In archaea, the 20S is composed of homo-heptameric α- and β-rings, and PAN (Proteasomal Activator Nucleotidase), a homohexamer proteasomal ATPase, is the RP found in many species. Unfolded substrates enter the chamber through a narrow pore in the center of α-rings, where N-termini of α-subunits form a gate to impede unregulated access to the proteolytic chamber. We designed and assembled in vitro various asymmetric archaea 20S, in which one of the two α-rings contains a point mutation, K66A, which prevents RP binding to the α-ring. Our studies reveal that, upon binding of a RP with a conserved C-terminal HbYX motif to one α-ring, the gate of the opposite α-ring opens allosterically, resulting in similar proteolytic activities of 20S singly capped and doubly capped with PAN.

The second activator is heptameric PA26 with the point mutation E102A and the last eight C-terminal residues replaced with the last eight C-terminal residues from PAN (with HbYX motif), which we named PA26PANc. The point mutation E102A abolishes a specific interaction between the so-called activation loop of PA26 with a reverse turn loop in the 20S α-subunit, thus abolishing the capability of PA26 to activate 20S proteasomes by opening its gate. Instead, the HbYX motif from the PAN C-terminus placed at the heptameric PA26PANc C-termini performs gate opening. PA26PANc activates the CP particle in the same manner as PAN, except that it symmetrically engages the 7-fold symmetric α-ring, and thus avoids a symmetry mismatch between the α-ring and the activator. We first determined the structure of PA26PANc-αWTββαK66A to resolutions of 2.9 Å without LFP substrate and 3.4 Å with LFP. In both our structures (with and without LFP), the distal α-ring, that without an activator, also shows features that match an open gate, with all N-termini moved away from the pore and pointing upwards. However, unlike the proximal gate, there is no rotation of distal α-subunits. Rather, the conformation of this α-ring matches well with that in the crystal structure of archaeal 20S proteasome in complex with PA26 (PDB: 1YAR20), except that the gate is in an open conformation. The surprising observation that binding of PA26PANc to the proximal α-ring opens the gate of the distal α-ring is consistent with allosteric action.

>[14x]TTTVGITLKDAVIMATERRVTMENFIMHKNGKKLFQIDTYTGMTIAGLVGDAQVLVRYMKAELELYRLQRRVNMPIEAVATLLSNMLNQVKYMPYMVQLLVGGIDTAPHVFSIDAAGGSVEDIYASTGSGSPFVYGVLESQYSEKMTVDEGVDLVIRAISAAKQRDSASGGMIDVAVITRKDGYVQLPTDQIESRIRKLGLIL;>AYDRAITVFSPDGRLFQVEYAREAVKKGSTALGMKFANGVLLISDKKVRSRLIEQNSIEKIQLIDDYVAAVTSGLVADARVLVDFARISAQQEKVTYGSLVNIENLVKRVADQMQQYTQYGGVRPYGVSLIFAGIDQIGPRLFDCDPAGTINEYKATAIGSGKDAVVSFLEREYKENLPEKEAVTLGIKALKSSLEEGEELKAPEIASITVGNKYRIYDQEEVKKFL[7x];>[7x]KRAALIQNLRDSYTETSSFAVIEEWAAGTLQEIEGIAKAAVEAHGTIRNSTYGRAQAEKSPEQLLGVLQRYQDLCHNVYCQAETIRTVIAIRIPEHKEADNLGVAVQHAVLKVIDELEIKTLGSGEKSGSGGAPTPIGMYALREYLSARSTVEDKLLGSVDAESGKTKGGSQSPSLLLELRQIDADFMLKVELATTHLSTMVRAVINAYLLNWKKLIQPRGGHLDVLYR;>YDRAITVFSPDGRLFQVEYAREAVKKGSTALGMKFANGVLLISDKKVRSRLIEQNSIEAIQLIDDYVAAVTSGLVADARVLVDFARISAQQEKVTYGSLVNIENLVKRVADQMQQYTQYGGVRPYGVSLIFAGIDQIGPRLFDCDPAGTINEYKATAIGSGKDAVVSFLEREYKENLPEKEAVTLGIKALKSSLEEGEELKAPEIASITVGNKYRIYDQEEVKKFL[7x]>ARKKYMEISLLTDIGQRRSNNQDFINQFENKAGVPLIILADGMGGHRAGNIASEMTVTDLGSDWAETDFSELSEIRDWMLVSIETENRKIYELGQSDDYKGMGTTIEAVAIVGDNIIFAHVGDSRIGIVRQGEYHLLTSDHSLVNELVKAGQLTEEEAASHPQKNIITQSIGQANPVEPDL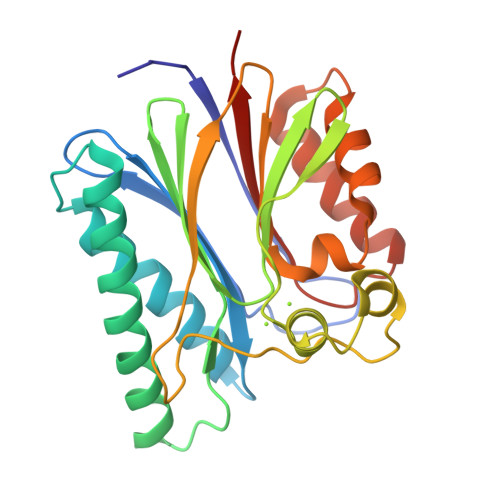GVHLLEEGDYLVVNSDGLTNMLSNADIATVLTQEKTLDDKNQDLITLANHRGGLDNITVALVYVESEAV[4x]> VCSLDNGDCDQFC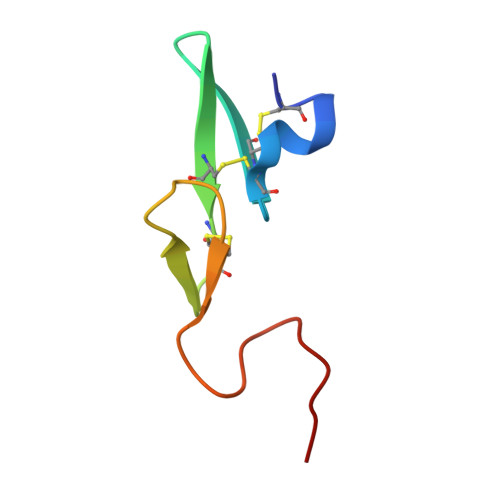HEEQNSVVCSCARGYTLADNGKACIPTGPYPCGKQTLE>[2x]MSLQTRKQREDAKREAWKKERQEKKALEAQQDSVSYVQAINALKNGSFVLEADNVVF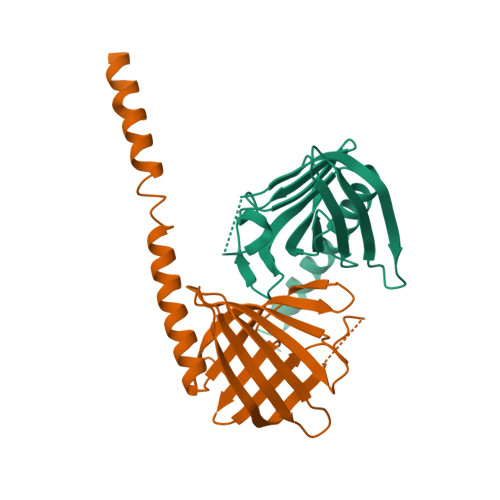RNGIMRFVSSNTNYVEVNDGQGIIQTAFTNFVYNWSPNGLGGVTVQGNVNGISMRQDKDGNVYYNYGINGIAVSATVSIVLTGGTNQASVTINPNFSGNTLTMNGYLVPYNEGHHHHHH> SDSLSKSPENWMSKLDDGKHLTEINIPGSHDSGSFTLKDPVKSVWAKTQDKDYLTQMKSGVRFFDIRGRASADNMI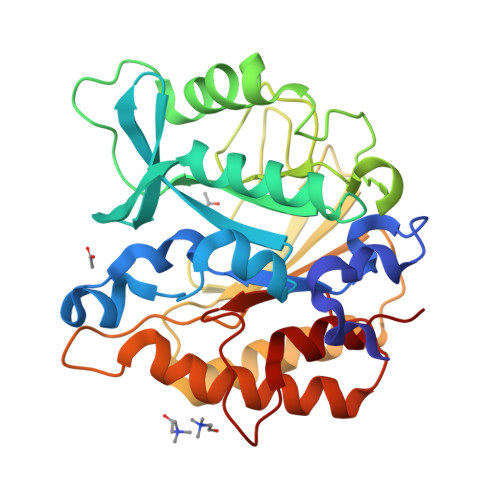SVHHGMVYLHHELGKFLDDAKYYLSAYPNETIVMSMKKDYDSDSKVTKTFEEIFREYYYNNPQYQNLFYTGSNANPTLKETKGKIVLFNRMGGTYIKSGYGADTSGIQWADNATFETKINNGSLNLKVQDEYKDYYDKKVEAVKNLLAKAKTDSNKDNVYVNFLSVASGGSAFNSTYYYASYINPEIAKTIKANGKARTGWLIVDYAGYTWPGYDDIVSEIIDSNKL>MTHLFEGVGVALTTPFTNNKVNIEALKTHVNFLLENNAQAIIVNGTTAESPTLTTDEKERILKTVIDLVDKRVPVIAGTGTNDTEKSIQASIQAKALGADAIMLITPYYNKTNQRGLVKHFEAIADAVKLPVVLYNVPSRTNMTIEPETVEILSQHPYIVALKDATNDFEYLEEVKKRIDTNSFALYSGNDDNVVEYYQRGGQGVISVIANVIPKEFQALYDAQQSGLDIQDQFKPIGTLLSALSVDINPIPIKALTSYLGFGNY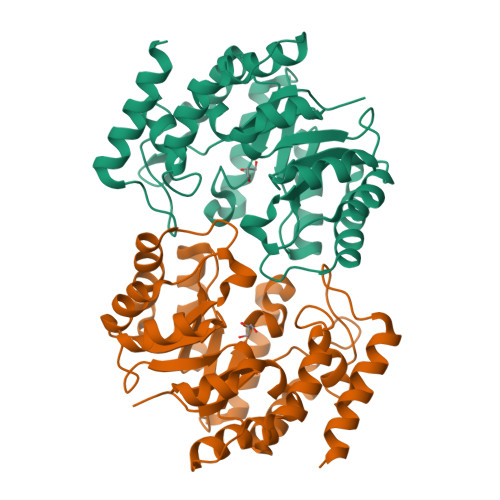ELRLPLVSLEDTDTKVLRETYDTFKAGENE[2x]>[2x]GHMSPNYDKWEMERTDITMKHKLGGGQYGEVYEGVWKKYSLTVAVKTLKEDTMEVEEFLKEAAVMKEIKHPNLVQLLGVCTREPPFYIITEFMTYGNLLDYLRECNRQEVNAVVLLYMATQISSAMEYLEKKNFIHRDLAARNCLVGENHLVKVADFGLSRLMTGDTYTAHAGAKFPIKWTAPESLAYNKFSIKSDVWAFGVLLWEIATYGMSPYPGIDLSQVYELLEKDYRMERPE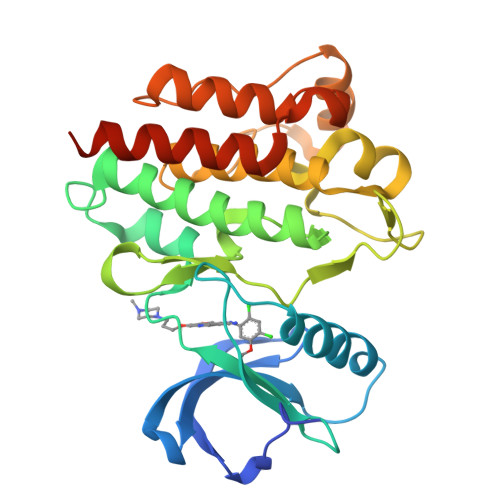GCPEKVYELMRACWQWNPSDRPSFAEIHQAFETMFQESSISDEVEKELGK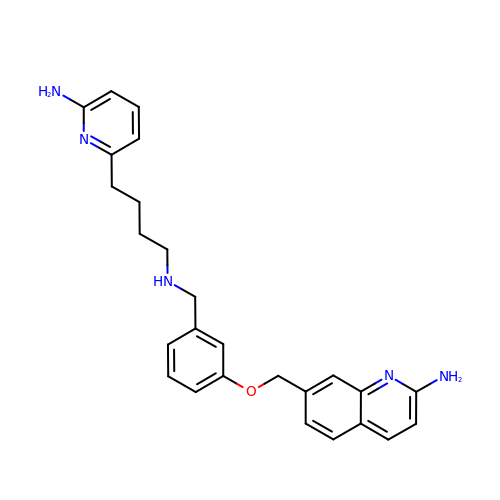7-{[3-({[4-(6-aminopyridin-2-yl)butyl]amino}methyl)phenoxy]methyl}quinolin-2-amine | C26 H29 N5 O | QYKBESYQSCLLGR-UHFFFAOYSA-N>[4x]MGLSLPKEKGLILCLWSKFCRWFQRRESWAQSRDEQNLLQQKRIWESPLLLAAKDNDVQALNKLLKYEDCKVHQRGAMGETALHIAALYDNLEAAMVLMEAAPELVFEPMTSELYEGQTALHIAVVNQNMNLVRALLARRASVSARATGTAFRRSPCNLIYFGEHPLSFAACVNS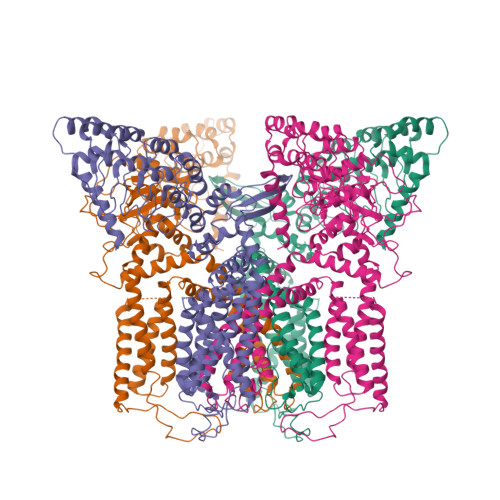EEIVRLLIEHGADIRAQDSLGNTVLHILILQPNKTFACQMYNLLLSYDRHGDHLQPLDLVPNHQGLTPFKLAGVEGNTVMFQHLMQKRKHTQWTYGPLTSTLYDLTEIDSSGDEQSLLELIITTKKREARQILDQTPVKELVSLKWKRYGRPYFCMLGAIYLLYIICFTMCCIYRPLKPRTNNRTSPRDNTLLQQKLLQEAYMTPKDDIRLVGELVTVIGAIIILLVEVPDIFRMGVTRFFGQTILGGPFHVLIITYAFMVLVTMVMRLISASGEVVPMSFALVLGWCNVMYFARGFQMLGPFTIMIQKMIFGDLMRFCWLMAVVILGFASAFYIIFQTEDPEELGHFYDYPMALFSTFELFLTIIDGPANYNVDLPFMYSITYAAFAIIATLLMLNLLIAMMGDTHWRVAHERDELWRAQIVATTVMLERKLPRCLWPRSGICGREYGLGDRWFLRVEDRQDLNRQRIQRYAQAFHTRGSEDLDKDSVEKLELGCPFSPHLSLPMPSVSRSTSRSSANWERLRQGTLRRDLRGIINRGLEDGESWEYQILVPRGSAAAWSHPQFEK> MYYGISQFSEAYNKILRNSSSHSSCQLVIFVSCLNIDALCATKMLSLLFKKQLVQSQIVPIFGYSELRRHYSQLDDNINSLLLVGFGGVIDLEAFLEIDPQEYVIDTDEKSGEQSFRRDIYVLDAHRPWNLDNIFGSQIIQCFDDGTVDDTLGEQKEAYYKLLELDEESGDDELSGDENDNNGGDDEATDADEVTDEDEEDEDETISNKRGNSSIGPNDLSKRKQRKKQIHEYEGVLEEYYSQGTTVVNSISAQIYSLLSAIGETNLSNLWLNILGTTSLDIAYAQVYNRLYPLLQDEVKRLTPSSRNSVKTPDTLTLNIQPDYYLFLLRHSSLYDSFYYSNYVNAKLSLWNENGKKRL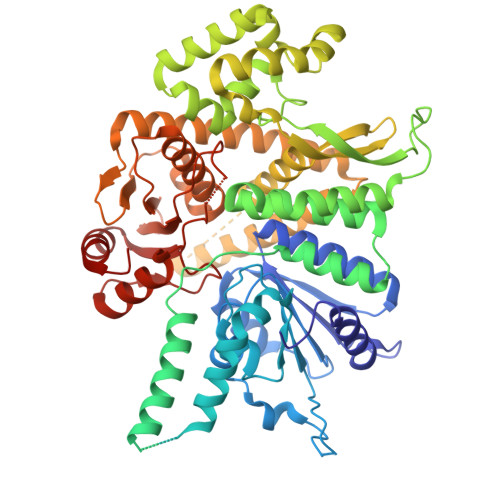HKMFARMGIPLSTAQETWLYMDHSIKRELGIIFDKNLDRYGLQDIIRDGFVRTLGYRGSISASEFVEALTALLEVGNSTDKDSVKINNDNNDDTDGEEEEDNSAQKLTNLRKRWVSNFWLSWDALDDRKVELLNRGIQLAQDLQRAIFNTGVAILEKKLIKHLRIYRLCVLQDGPDLDLYRNPLTLLRLGNWLIECCAESEDKQLLPMVLASIDENTDTYLVAGLTPRYPRGLDTIHTKKPILNNFSMAFQQITAETDAKVRIDNFESSIIEIRREDLSPFLEKLTLSGLL Twenty-S rRNA accumulation 1 (Tsr1) is an essential 40S subunit biogenesis factor with homology to characterized GTPases. Tsr1 is a key nucleo-cytoplasmic pre-40S ribosome biogenesis factor that is essential for the final maturation of 20S rRNA to 18S rRNA91014. However, Tsr1 lacks all the conserved motifs required for guanine nucleotide binding and GTP hydrolysis, and is therefore a structural mimic of translational GTPases rather than a functional enzyme. Since Tsr1 is not catalytically active these data suggest that, rather than acting as a molecular switch, Tsr1 is a molecular gatekeeper that must be removed before key sites can be accessed to catalyse the final stages of pre-40S maturation.

We reasoned that this segment might hinder crystallization, so we generated a ‘loop-out' mutant (Tsr1Δloop), in which residues 410–476 of Tsr1 were replaced with a short glycine- and serine-rich sequence. A further deletion of sequence predicted to be natively unstructured at the N terminus (Tsr1ΔNΔloop) improved diffraction quality, generating native crystals that diffracted to 3.6 Å. We found that Tsr1ΔNΔloop complements loss of wild-type Tsr1 in yeast, showing that the N terminus and acidic loop are dispensable for Tsr1 function in vivo. Comparison of the four molecules in the asymmetric unit shows only limited differences between them (root mean squared deviation (r.m.s.d.) values range from 0.9 to 1.1 Å) suggesting that the overall domain arrangement of Tsr1 is fixed. Tsr1 is characterized by four domains that pack together to form a chalice-like structure. The N-terminal domain (domain I) has a small GTPase-like fold. The second, third and fourth domains (II–IV) are β-barrels. Domain II has a large insertion segment that wraps around the centre of the molecule. The first and last β-strands of domain IV form an extended, two-stranded β-sheet, placing domain IV at the periphery of the structure and burying the C terminus of the protein in the core of the protein between domains I and III. Comparison of Tsr1 with EF-Tu shows that Tsr1 has a domain arrangement similar to EF-Tu in its GTP-bound, active form.

>[4x]MKHHHHHHSAGLEVLFQGPDSMDKQVSKLQRKNKAKQLRAQRILDSIENRKLFEGKNGAAKIITIVPLVNDLDPLDILYKLLKCADDEGIMVQEVDSKRIFNVHIKKFKSNLKIIIPDMTNFLNILDCAKVADFVVFGLSGVQEVDEEFGEQIIRALELQGIASYIGVISNLSAVHEKEKFQLDVKQSLESYFKHFFPSEERVYNLEKNSDALNVLRTLCQRLPRSINWRDNRGYVVADFVDFVETSPDSGDLVIEGTVRGIGFNANRLVHIPDFGDFQLNKIEKISESSQKRKIIKEKATDSLSLELDLQTVFESNMNRDTLDEYAPEGTEDWSDYDEDFEYDGLTTARYDDHGFLPGREQTSKKAAVPKGTSDYQAKWYLDDVIPSSGSSKEDREFPDEIELEPSESAIERLKRYRGLKNLYNCDWQVDEKDPSSPAEWKRLLRIGNYKNTKNRIIKETKNEAQAIAGDRIRMFIRFPKFLLEKIQDPKQLLFAVYGLLLHEHKNAVVNFSLQRWEQYDKPVPSQEPIVVQYGVRRYTIQPLFSQGSNSPNNVHKYERFLHPDTVSVATCIAPVDFTQSPAIFFKPSPTDAKNIELIGHGTFLNADHSRILAKRAILTGHPFRFHKTVVTVRYMFFRPEDVEWFKSIPLFTKSGRSGFIKESLGTHGYFKATFDGKLSAQDVVAMSLYKRMWPMPSLPWNGM Bacterial multiheme cytochromes (MHCs) attract much attention for their contributions to extracellular electron transfer whereby electrons are exchanged across the cell boundary and consequently between internal enzymes and external redox partners. These processes evolved to allow the capture of electrons for anabolic reactions and the release of electrons from internal oxidation during anaerobic respiration. Thus, we investigated whether amber suppression in MR-1 could produce ncAA-containing MHCs and, specifically, variants of the MtrC protein, which contains ten c-type hemes. MtrC is found on the outer surface of MR-1 cells. MR-1 cells typically present MtrC tightly bound to the external face of the outer membrane spanning the MtrAB porin-cytochrome complex.

The structure of wtMtrC was inspected to identify surface residues that might be changed to ncAAs with limited effect on the MtrC structure. Residue A293 in Domain II and E344 and A430 in Domain III were chosen, Figure 2C. Thus, site-specific replacement of MtrC surface residues with BocK has no discernible impact on the protein structure. By contrast, there was no detectable FMN reduction for ΔmtrC/omcA MR-1 cells cultured in the absence of wtMtrC. Cells from cultures augmented by MtrC344BocK and MtrC430BocK also displayed FMN reduction rates comparable to those of MR-1, Figure 5C. Thus, our results indicate that MtrC344BocK and MtrC430BocK retain the structure and redox activity of wtMtrC. A crystal structure of the homologous MtrCAB complex purified from Shewanella baltica OS18542 shows that MtrC Domain III, which contains residues 344 and 430, makes no contribution to the binding with MtrAB. This is consistent with the ability of wtMtrC, MtrC344BocK, and MtrC430BocK to restore FMN reduction activity to ΔmtrC/omcA MR-1 cells by associating with MtrAB in the outer membrane.

> MKFKLNLITLALLANTGLAVAADGGSDGNNGNDGSDGGEPAGSIQTLNLDITKVSYENGAPMVTVFATNEADMPVIGLANLEIKKALQLIPEGATGPGNSANWQGLGSSKSYVDNKNGSYTFKFDAFDSNKVFNAQLTQRFNVVSAAGKLADGTTVPVAEMVEDFDGQGNAPQYTKNIVSHEVCASCHVEGEKIYHQATEVETCISCHTQEFADGRGKPHVAFSHLIHNVHNANKAWGKDNKIPTVAQNIVQDNCQVCHVESDMLTEAKNWSRIPTMEVCSSCHVDIDFAAGKGHSQQLDNSNCIACHNSDWTAELHTAKTTATKNLINQYGIETTSTINTETKAATISVQVVDANGTAVDLKTILPKVQRLEIITNVGPNNATLGYSGKDSIFAIKNGALDPKATINDAGKLVYTTTKDLKLGQNGKDSDTAFSFVGWSMCSSEGKFVDCADPAFDGVDVTKYTGMKADLAFATLSGKAPSTRHVDSVNMTACANCHTAEFEIHKGKQHAGFVMTEQLSHTQDANGKAIVGLDACVTCHTPDGTYSFANRGALELKLHKKHVEDAYGLIGGNCASCHSDFNLESFKKKGALNTAAAADKTGLYSTPITATCTTCHTVGSQYMVHTKETLESFGAVVDGTKDDATSAAQSETCFYCHTPTVADHTKVKMSAWSHPQFEK> MDPKISEMHPALRLVDPQIQLAVTRMENAVG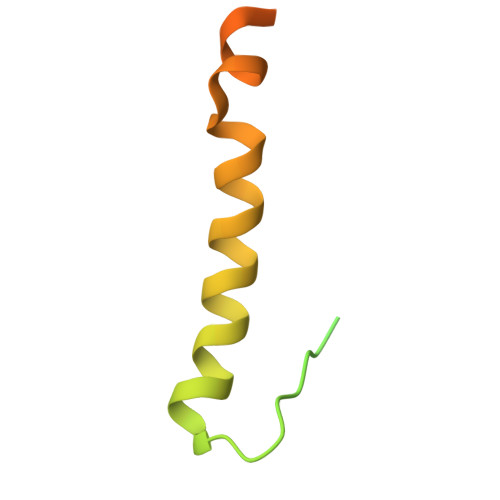RDQNNVGPKVYPIILRLGSPLSLNMARKTLNSLEDKAFQLTPIAVQMTKLATTEELPDEFVVVTVK> MQWIRGGSGMLITGDSIVSAEAVWDHVTMANRELAFKAGDVIKVLDASNKDWWWGQIDDEEGWFPASFVRLWVNQEDGVEEGPSDVQNGHLDPNSDCLCLGRPLQNRDQMRANVINEIMSTERHYIKHLK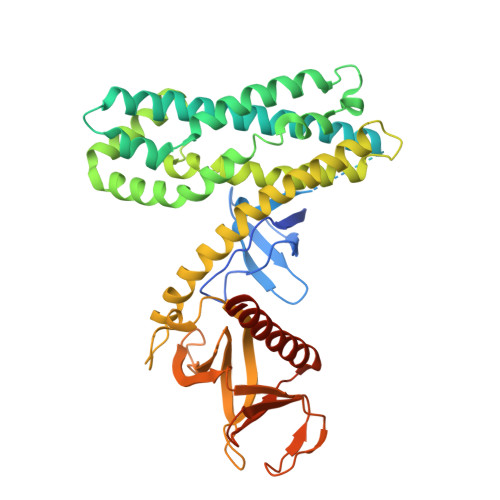DICEGYLKQCRKRRDMFSDEQLKVIFGNIEDIYRFQMGFVRDLEKQYNNDDPHLSEIGPCFLEHQDGFWIYSEYCNNHLDACMELSKLMKDSRYQHFFEACRLLQQMIDIAIDGFLLTPVQKICKYPLQLAELLKYTAQDHSDYRYVAAALAVMRNVTQQINERKRRLENIDKIAQWQASVLDWEGDDILDRSSELIYTGEMAWIYQPYGRNQQRVFFLFDHQMVLCKKDLIRRDILYYKGRIDMDKYEVIDIEDGRDDDFNVSMKNAFKLHNKETEEVHLFFAKKLEEKIRWLRAFREERKMVQEDEKIGFEISENQKRQAAMTV> QLLQPLPAEIKGTKLLAHWASGATITCIPESFLEDEQPIKKTLIKTIHGEKQQNVYYVTFKVKGRKVEAEVIASPYEYILLSPTDVPWLTQQPLQLTILVPLQEYQEKILSKTALPEDQKQQLKTLFVKYDNLWQHWENQVGHRKIRPHNIATGDYPPRPQKQYPINPKAKPSIQIVIDDLLKQGVLTPQNSTMNTPVYPVPKPDGRWRMVLDYREVNKTIPLTAAQNQHSAGILATIVRQKYKTTLDLANGFWAHPITPESYWLTAFTWQGKQYSWTRLPQGFLNSPALFTADVVDLLKEIPNVQVYVDDIYLSHDDPKEHVQQLEKVFQILLQAGYVVSLKKSEIGQKTVEFLGFNITKEGRGLTDTFKTKLLNITPPKDLKQLQSILGLLNFARNFIPNFAELVQPLYNLIASAKGKYIEWSEENTKQLNMVIEALNTASNLEERLPEQRLVIKVNTSPSAGYVRYYNETGKKPIMYLNYVFSKAELKFSMLEKLLTTMDKALIKAMDLAMGQEILVYSPIVSMTKIQKTPLPERKALPIRWITWMTYLEDPRIQFHYDKTLPELKHIPDVYTSSQKPVKHPSQYEGVFYTDGSAIKSPDPTKSNNAGMGIVHATYKPEYQVLNQWSIPLGNHTAQMAEIAA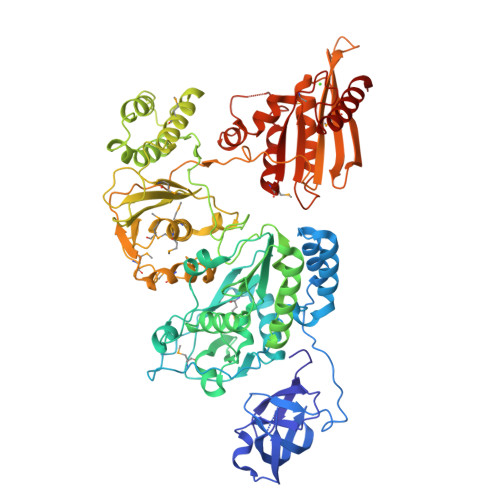VEFACKKALKIPGPVLVITDSFYVAESANKELPYWKSNGFVNNKKKPLKHISKWKSIAECLSMKPDITIQHEKGHQPTNTSIHTEGNALADKLATQGSYVVN1-(4-{[(3R)-3-AMINO-5-{[(Z)-AMINO(IMINO)METHYL](METHYL)AMINO}PENTANOYL]AMINO}-2,3,4-TRIDEOXY-D-ERYTHRO-HEX-2-ENOPYRANURONOSYL)-4-HYDROXYPYRIMIDIN-2(1H)-ONE 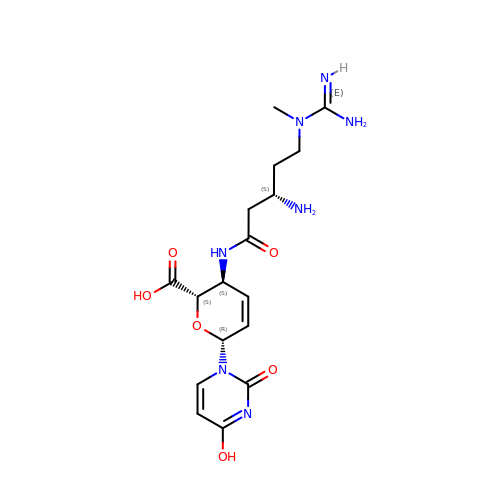| C17 H25 N7 O6 | REIIQZAQCCFGIJ-ZNIXKSQXSA-N> MSGSNMGYYDVLAGLSALEKSSQVVFSATELQQLTQQSHAT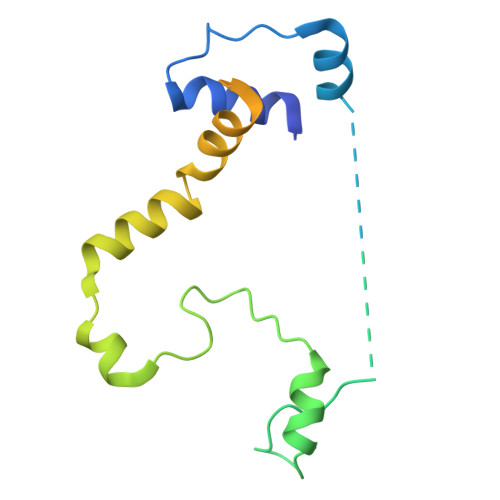DKGIEGSENSKAKVSKPKRVAVHGYLGGKVSLADAAQVEYEVGHSLLGSYVPRQQLEALSSVDFSHHFHRTLECKAALETHDVFLAGAGQLSLPFQSHIESPRNSEAKRKRKVIICKRCQSRFIGSHRRSQLREHACVD>[6x]MAKSTTFFISLTLPFLLLSVVTATYYQSMSPTVLGFQEEKFTHLHFYFHDVVTGPKPSMVIVAEPNGKAKNSLPFGTVVAMDDPLTVGPESDSKLVGKAQGIYTSISQEEMGLMMVMTMAFSDGEFNGSTLSILARNMIMSEPVREMAIVGGTGAFRFARGYAQAKFYSVDFTKGDAIVEYDIFVFHYKGELNSKLEGKPIPNPLLGLDSTRTGHHHHHH

Described herein are the 3D structures of two stereoselective pterocarpan-forming DPs from pea and licorice, which preferentially produce either (+)- or (–)-medicarpin, depending on the substrate. We describe that pterocarpan synthases, containing dirigent-like domains, initially engender mono-QM formation from their chiral substrates, this being followed by intramolecular cyclization (C–O bond formation) to afford entry into the pterocarpan natural product (phytoalexin) class. GePTS1 and PsPTS1, in solution, exist mainly as trimers (∼68.0 kDa), with (because of association/aggregation) a small amount of higher-molecular weight entities also being evident (roughly corresponding to 410–500 kDa). The entrance to the putative active site of the GePTS1 and PsPTS1 monomers is located at the end of the barrel opposite the N and C termini.

The GePTS1 structure was solved by molecular replacement at 2.6 Å resolution. Six independent DP monomer molecules, labeled A–F, were located in the crystallographic asymmetric unit, arranged as a dimer of trimers. The buried surface area between the two trimers is small, and the biologically active form in solution is presumed to be a trimer, as confirmed by GPC analysis. The GePTS1 monomer is an eight-stranded antiparallel β-barrel comprised of two curved anti-parallel sheets formed by strands β1′, β2, β3, β4, β5, and β6′ (designated sheet I) and β6, β7, β8, and β1 (designated sheet II) that contact each other only slightly at the β1′-β8 and β5-β6′ interfaces. Currently, the GePTS1 structure is the only one that shows the trimer without requiring it to be generated by crystallographic symmetry, being found as a dimer of trimers in the asymmetric unit. For example, in GePTS1, the cavity volumes range between 350 and 500 Å3 (calculated with ICM-Pro) and are lined by predominantly aromatic and hydrophobic residues and two aspartate residues (Asp50 and Asp83). The roughly cylindrical active-site cavity is long and narrow (around 7 Å diameter) and nearly parallel to the 3-fold symmetry axis of the trimer, where Tyr181 sits at the base of the tunnel with its hydroxyl group projecting along the tunnel axis. The conserved polar residues in the active site of GePTS1—Asp50, Asp83, Tyr103, Asn137, Arg145, and Tyr181—are likely to facilitate this mechanism. All four GePTS1 mutants, when subjected to comprehensive kinetic analysis, displayed large reductions in catalytic turnover.>[2x]GAAUUGCGGGAAAGGGGUCAACAGCCGUUCAAUACCAAGUCUCAGGGGAAACUUU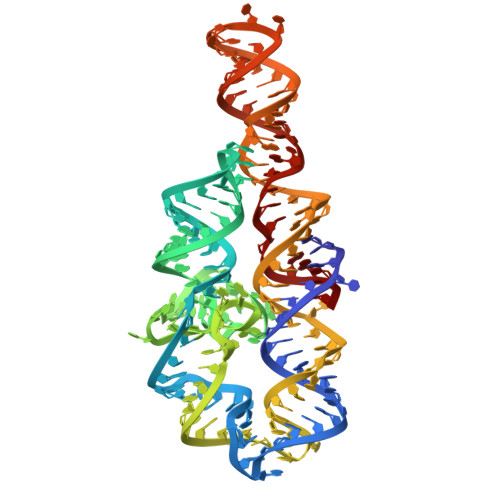GAGAUGGCCUUGCAAAGGGUAUGGUAAAAAAGCUGACGGACAUGGUCCUAACCACGCAGCCAAGUCCUAAGUCAACAGAUCUUCUGUUGAUAUGGAUGCAGUUC>HHHHHHSLVPRGSPSRSVILTGNSSLCPISGWAIYSKDNGIRIGSKGDVFVIREPFISCSHLECRTFFLTQGALLNDKHSNGTVKDRSPYRTLMSCPVGEAPSPYNSRFESVAWSASACHDGMGWLTIGISGPDNGAVAVLKYNGIITDTIKSWRNNILRTQESECAC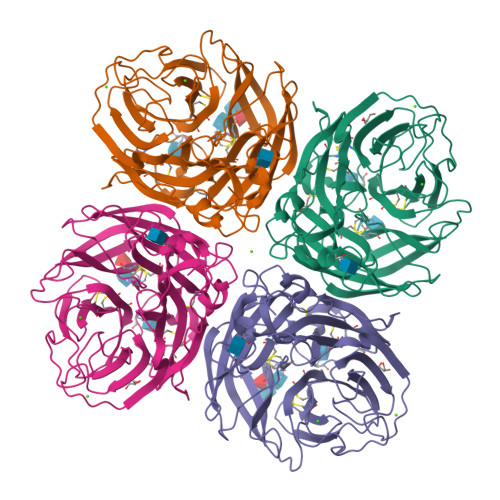VNGSCFTIMTDGPSNGQASYKILKIEKGKVTKSIELNAPNYHYEECSCYPDTGKVMCVCRDNWHGSNRPWVSFDQNLDYQIGYICSGVFGDNPRPNDGTGSCGPVSSNGANGIKGFSFRYDNGVWIGRTKSTSSRSGFEMIWDPNGWTETDSSFSVRQDIVAITDWSGYSGSFVQHPELTGLDCMRPCFWVELIRGQPKENTIWTSGSSISFCGVNSDTVGWSWPDGAELPFSIDK[8x]> GGSNYSADSGNTVYVGNIDPRITKEQLYELFIQINPVLRIKYPKDKVLQAYQ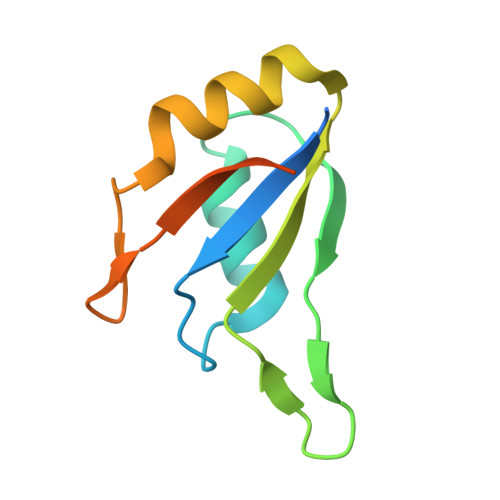GYAFIEFYNQGDAQYAIKIMNNTVRLYDRLIKVRQVTNSTGTTNLPSNIS>MSQFTLYKNKDKSSAKTYPYFVDVQSDLLDNLNTRLVIPLTPIELLDKKAPSH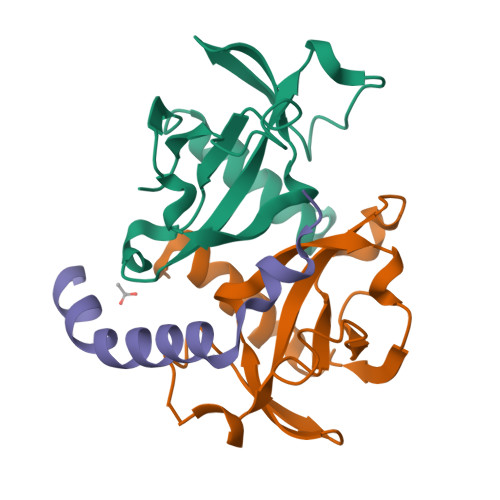LCPTIHIDEGDFIMLTQQMTSVPVKILSEPVNELSTFRNEIIAAIDFLITGI[2x];> RRLRAERWKAENQEGMAEVARFIEMNGSFADENRDW Unlike Cas9 and Cas12, Cas13 is an RNA-guided RNA endonuclease containing two HEPN (higher eukaryotes and prokaryotes nucleotide-binding) nuclease domains. Cas13bt3 (also known as Cas13X.1) was recently identified as a minimal Cas13 protein (775 residues) and used for RNA knockdown in mammalian cells. The crystal structure revealed that Cas13bt3 adopts a bilobed architecture consisting of the REC and NUC lobes, with the crRNA DR anchored in the REC lobe. The NUC lobe comprises the HEPN1 and HEPN2 domains, while the REC lobe consists of the Helical-1, Lid, and Helical-2 domains.

To clarify the crRNA-guided target RNA recognition and cleavage mechanisms of Cas13bt3, we determined the cryo-EM structure of dCas13bt3 in complex with a crRNA (61 nucleotides) and its complementary target RNA (25 nucleotides), at an overall resolution of 3.4 Å. The density was less clear for the NUC lobe as compared with the REC lobe, suggesting that the NUC lobe is relatively flexible in the ternary complex. Thus, we modeled the HEPN1/HEPN2 dimer structure in the binary complex into the density map as a single rigid body, except for a flexible loop in the HEPN2 domain (residues 703–729, referred to as an active site loop [ASL]), which was not resolved in the density map. The crRNA spacer (G20–U1) base pairs with the target RNA (A1–C20), while the terminal five base pairs (G21-C21–G25-C25) are disordered. The crRNA-target RNA duplex is bound to the groove formed by the Helical-1, Lid, HEPN1, and HEPN2 domains. Upon target RNA binding, the HEPN1 domain moves away from the REC lobe, with IDL1 serving as a pivot point. In contrast, in the ternary complex, the short a helix is melted and residues 582–608 form a continuous a helix. These structural rearrangements of the HEPN1 and HEPN2 domains result in the formation of a binding groove for the crRNA-target RNA duplex. A structural comparison between the binary and ternary complexes revealed that, whereas the ASL is ordered and covers the HEPN1 active site in the binary complex, it is disordered and the HEPN1 active site is accessible in the ternary complex. In the Cas13bt3-crRNA-target RNA ternary complex, the HEPN domains move away from the REC lobe, and thus, the ASL becomes more flexible and dissociates from the HEPN active site, thereby allowing the access of ssRNA substrates to the catalytic residues.

> GGMAQVSKQTSKKRELSIDEYQGARKWCFTIAFNKALVNRDKNDGLFVESLLRHEKYSKHDWYDEDTRALIKCSTQAANAKAEALANYFSAYRHSPGCLTFTAEDELRTIMERAYERAIFECRRRETEVIIEFPSLFEGDRITTAGVVFFVSFFVERRVLDRLYGAVSGLKKNEGQYKLTRKALSMYCLKDSRFTKAWDKRVLLFRDILAQLGRIPAEAYEYYHGEQGDKKRANDNEGTNPKRHKDKFIEFALHYLEAQHSEICFGRRHIVREEAGAGDEHKKHRTKGKVVVDFSKKDEDQSYYISKNNVIVRIDKNAGPRSYRMGLNELKYLVLLSLQGKGDDAIAKLYRYRQHVENILDVVKVTDKDNHVFLPRFVLEQHGIGRKAFKQRIDGRVKHVRGVWEKKKAATNEMTLHEKARDILQYVNENCTRSFNPGEYNRLLVCLVGKDVENFQAGLKRLQLAERIDGRVYSIFAQTSTINEMHQVVCDQILNRLCRIGDQKLYDYVGLGKKDEIDYKQKVAWFKEHISIRRGFLRKKFWYDSKKGFAKLVEEHLESGGGQRDVGLDKKYYHIDAIGRFEGANPALYETLARDRLCLMMAQYFLGSVRKELGNKIVWSNDSIELPVEGSVGNEKSIVFSVSDYGKLYVLDDAEFLGRICEYFMPHEKGKIRYHTVYEKGFRAYNDLQKKCVEAVLAFEEKVVKAKKMSEKEGAHYIDFREILAQTMCKEAEKTAVNKVARAFFAHHLKFVIDEFGLFSDVMKKYGIEKEWKFPVK> MNLPTAQEVQGLMARYIELVDVGDI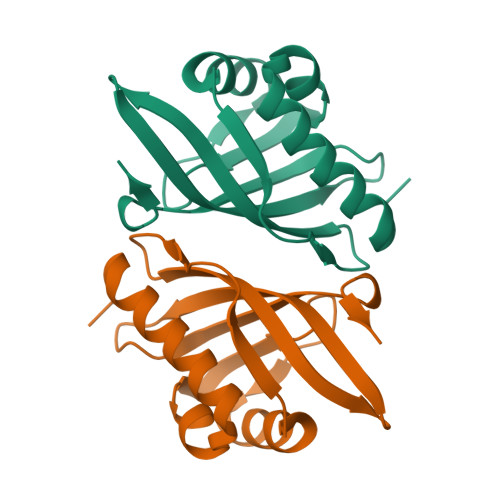EAIVQMFADDATVEDPFGQPPIHGREQIAAFFRQGLGGGKVRACLTGPVRASHNGCGAMPFRVEMVWNGQPCALDVIDVMRFDEHGRIQTMQAYWSEVNLSVREPQ ARABINO-FLAVIN-ADENINE DINUCLEOTIDE | C27 H33 N9 O15 P2 | 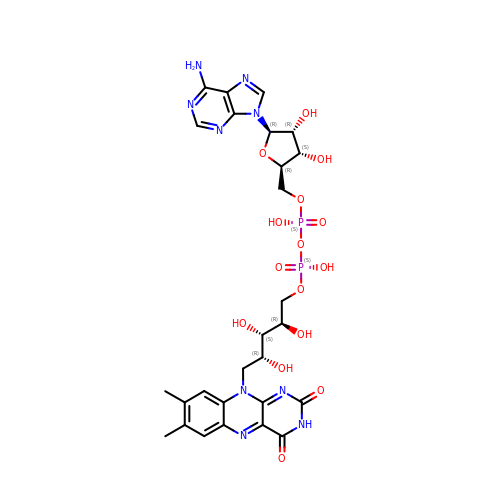VWWQXMAJTJZDQX-WCVIGVMNSA-N>[6x]PARPAHPLDPLSTAEIKA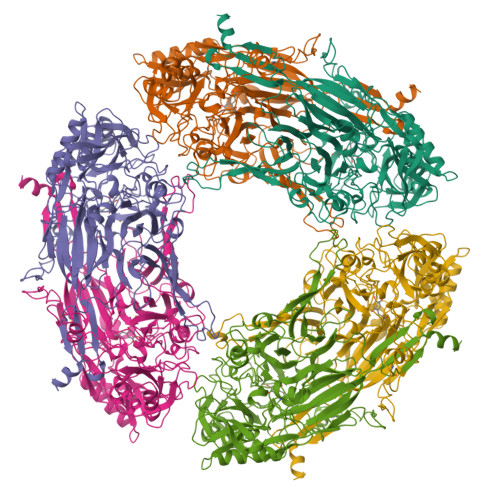ATNTVKSYFAGKKISFNTVTLREPARKAYIQWKEQGGPLPPRLAYYVILEAGKPGVKEGLVDLASLSVIETRALETVQPILTVEDLCSTEEVIRNDPAVIEQCVLSGIPANEMHKVYCDPWTIGYDERWGTGKRLQQALVYYRSDEDDSQYSHPLDFCPIVDTEEKKVIFIDIPNRRRKVSKHKHANFYPKHMIEKVGAMRPEAPPINVTQPEGVSFKMTGNVMEWSNFKFHIGFNYREGIVLSDVSYNDHGNVRPIFHRISLSEMIVPYGSPEFPHQRKHALDIGEYGAGYMTNPLSLGCDCKGVIHYLDAHFSDRAGDPITVKNAVCIHEEDDGLLFKHSDFRDNFATSLVTRATKLVVSQIFTAANYEYCLYWVFMQDGAIRLDIRLTGILNTYILGDDEEAGPWGTRVYPNVNAHNHQHLFSLRIDPRIDGDGNSAAACDAKSSPYPLGSPENMYGNAFYSEKTTFKTVKDSLTNYESATGRSWDIFNPNKVNPYSGKPPSYKLVSTQCPPLLAKEGSLVAKRAPWASHSVNVVPYKDNRLYPSGDHVPQWSGDGVRGMREWIGDGSENIDNTDILFFHTFGITHFPAPEDFPLMPAEPITLMLRPRHFFTENPGLDIQPSYAMTTSEAKRAV> MRGSHHHHHHGLVPRGSMIRTMLQGKLHRVKVTHADLHYEGSCAIDQDFLDAAGILENEAIDIWNVTNGKRFSVYAIAAERGSRIISVNGAAAHCASVGDIVIIASFVTM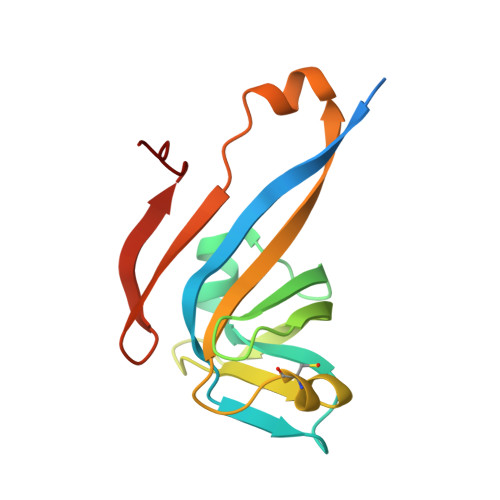PDEEARTWRPNVAYFEGDNEMKRTAKAIPVQVA>[2x]GPLGSDYIIKEKTVLLQKKDSEGFGFVLRGAKAQTPIEEFTPTPAFPALQYLESVDEGGVAWRAGLRMGDFLIEVNGQNVVKVGHRQVVNMIRQGGNTL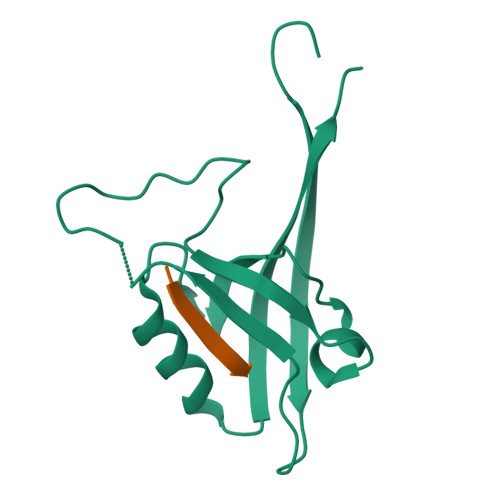MVKVVMVTRHPDM;>XEAQTRF[2x]> AEGKLNDELAKNKGKIPGLKIDQKIRGQMPERGWTEDDIKNTVSNGATGTSFDKRSPKKTPPDYLGRNDPATV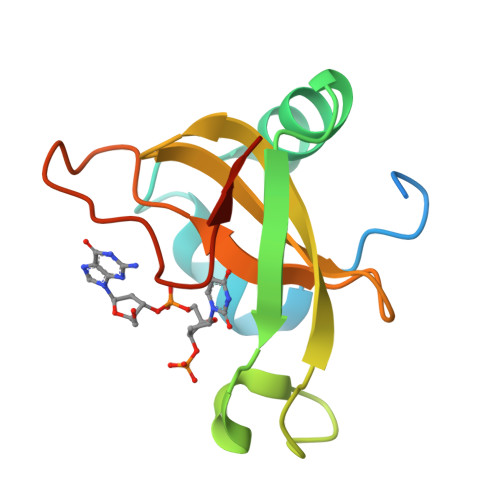YGSPGKYVVVNDRTGEVTQISDKTDPGWVDDSRIQWGNKNDQ>[2x]GPGSDKDCEMKRTTLDSPLGKLELSGCEQGLHEIIFLGKGTSAADAVEVPAPAAVLGGPEPLMQATAWLNAYFHQPEAIEEFPVPALHHPVFQQESFTR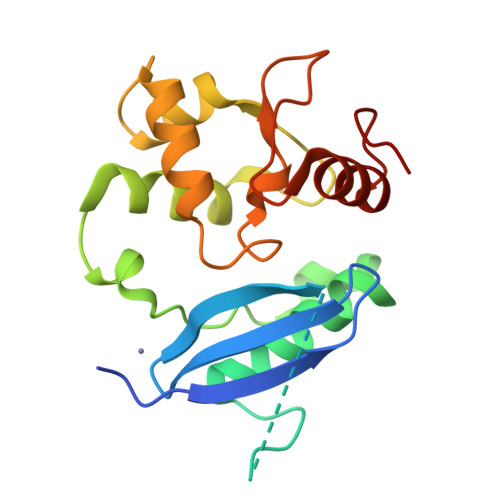QVLWKLLKVVKFGEVISYSHLAALAGNPAATAAVKTALSGNPVPILIPCHRVVQGDLDVGGYEGGLAVKEWLLAHEGHRLGKR3-(CARBOXYMETHYL)-4-ISOPROPENYLPROLINE 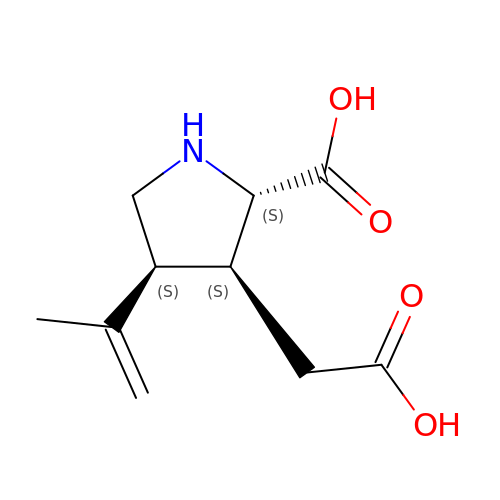| C10 H15 N O4 | VLSMHEGGTFMBBZ-OOZYFLPDSA-N> SGTTNTVAAYNLTWKSTNFKTILEWEPKPVNQ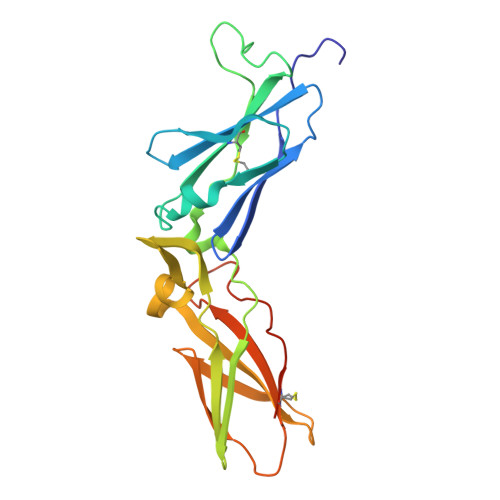VYTVQISTKSGDWKSKCFYTTDTECDLTDEIVKDVKQTYLARVFSYPAGNVESTGSAGEPLYENSPEFTPYLETNLGQPTIQSFEQVGTKVNVTVEDERTLVRRNNTFLSLRDVFGKDLIYTLYYWKSSSSGKKTAKTNTNEFLIDVDKGENYCFSVQAVIPSRTVNRKSTDSPVECMGQEKGEFRE>[2x]MRRLTAALCALTLLSTGAQAQTIKDFLAVAMKKWTAPFEPFQLIDNIYYVGTDGIAVYVIKTSQGLILMDTAMPQSTGMIKDNIAKLGFKVADIKLILNTHAHLDHTGGFAEIKKETGAQLV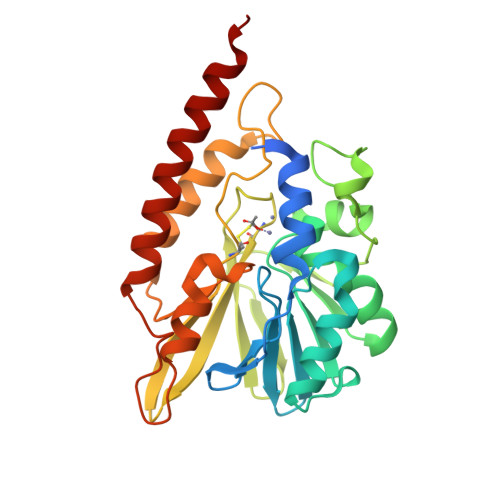AGERDKPLLEGGYYPGDEKNEDLAFPAVKVDRAVKEGDRVTLGDTTLTAHATPGHSPGCTSWEMTVKDGKEDREVLFFCSGTVALNRLVGQPTYAGIVDDYRATFAKAKAMKIDVLLGPHPEVYGMQAKRAEMKDGAPNPFIKPGELVTYATSLSEDFDKQLAKQTAALEKK>[2x]GEFKGLMAVGLAEHDKEAWGRLPFSLTIADISQDDEPLIYVNRAFEQMTGYSRSSVVGRNCRFLQGEKTDPGAVERLAKAIRNCEEVEETIYNYRADGEGFWNHLLMGPLEDQDEKCRY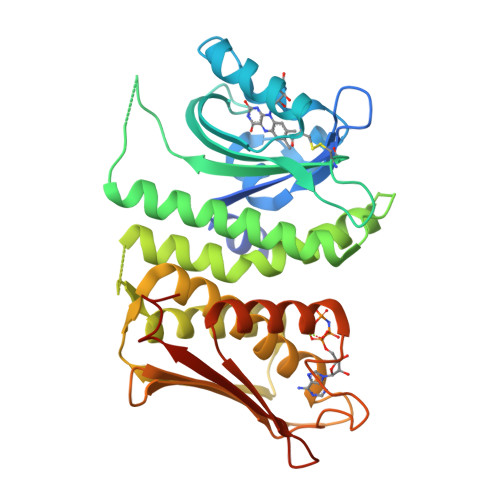FVGIQVDMGQSESPDRATELDRQLAEVQHRVKNHLAMIVSMIRIQSSQAGGVGSQFDSLSRRVEALQLLYQEMDIAGAAKATDKIIPLGAYLGRIASAINHIDGRGAIKVNVQADTVDVPVETAGRIGLLVSEVLTNALQHAFSDRASGVVQLRSSVMSGEQLRVTVEDDGRGIPEDCDWPNEGNLGSRIVRQLVQGLGAELNVTRGGTGTIVNIDIPLSQQKTLIADERTKD3-ethanoyl-~{N}-[2-fluoranyl-3-(1-methylpyrazol-4-yl)phenyl]-7-methoxy-indolizine-1-carboxamide | C22 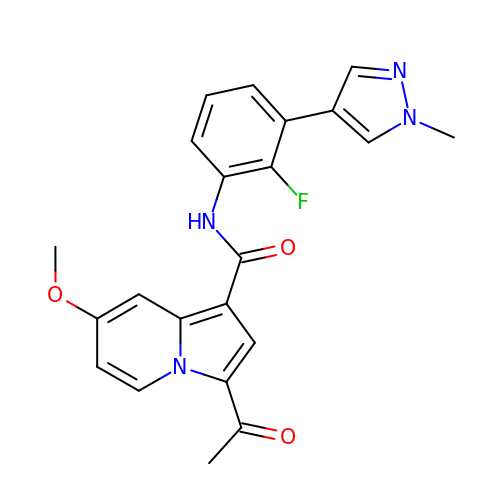H19 F N4 O3 | KERKYEVISFXSSG-UHFFFAOYSA-N>[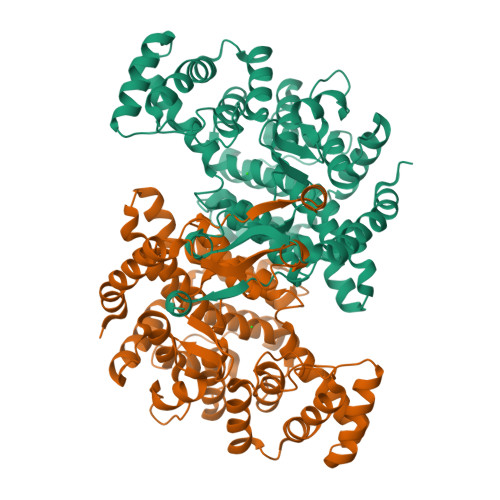6x]VQGQQSSLSNSVRWIQMQSSTDLDLKSQLQELIPEQQDRLKKLKSEHGKVQLGNITVDMVIGGMRGMTGLLWETSLLDPEEGIRFRGLSIPECQKVLPTAQSGAEPLPEGLLWLLLTGKVPSKEQVEALSKDLANRAAVPDYVYNAIDALPSTAHPMTQFASGVMALQVQSEFQKAYENGIHKSKFWEPTYEDCLNLIARVPVVAAYVYRRMYKNGDSIPSDKSLDYGANFSHMLGFDDEKVKELMRLYITIHSDHEGGNVSAHTGHLVGSALSDPYLSFAAALNGLAGPLHGLANQEVLLWIKSVVEECGEDISKEQLKEYVWKTLNSGKVIPGYGHGVLRNTDPRYVCQREFALKHLPDDPLFQLVSKLYEVVPPVLTELGKVKNPWPNVDAHSGVLLNHYGLTEARYYTVLFGVSRSLGICSQLIWDRALGLALERPKSVTMDWLEAHCKKASSA>[2x]GSHMSQSNRELVVDFLSYKLSQKGYSWSQFSDVEENRTEAPEGTESEMETPSAINGNPSWHLADSPAVNGATGHSSSLDAREVIPMAAVKQALREAGDEFELR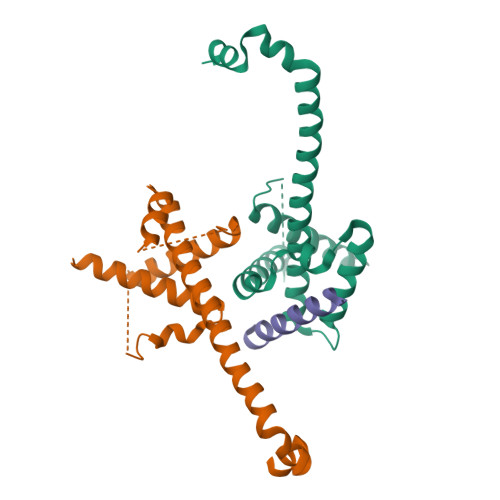YRRAFSDLTSQLHITPGTAYQSFEQVVNELFRDGVNWGRIVAFFSFGGALCVESVDKEMQVLVSRIAAWMATYLNDHLEPWIQENGGWDTFVELYGNNAAAESRKGQER;> EEQWAREIGAQLRRMADDLNAQYER> MATYYPPSSFHFLVEFTGIDAKNNDHEFQSVSGLSVDIDTEEFAEGGENRFKHKFPVKTKYPNLVLKRGV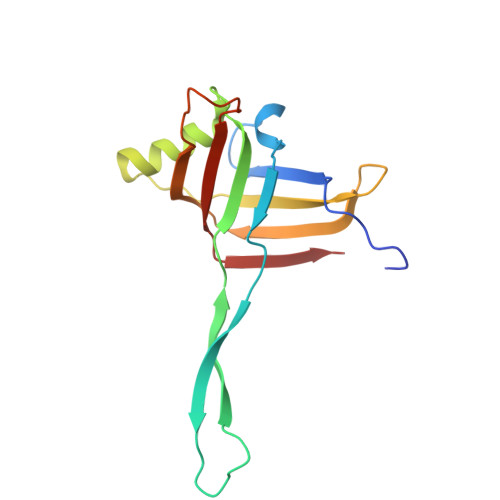LVDSKVISWCRDAIEDFEFKPIDLTVKLLNEEHQPLMTWNVVHAYPVKWSVEDFNAQESKMAIESVELSYNYFKTIV> APRKARTAFSDHQLNQLERSFERQKYLSVQDRMDLAAALNLTDTQVKTWYQNRRTKWKRQTAVG;> KKPRKARTAFSDHQLNQLERSFERQKYLSVQDRMDLAAALNLTDTQVKTWYQNRRTKWKRQTA

However, analyses of the formation of TF complexes on DNA have revealed that many TFs also bind together across the family boundaries, in a DNA-dependent or DNA-facilitated manner. Because the DNA-bound TFs are fixed at particular positions relative to each other, the contact surfaces required for cooperative DNA-facilitated binding are very small, and can evolve rapidly. We also generated an unseen test set by solving six structures that represent several TF–TF–DNA complexes bound to optimal DNA sequences. The structures included two BARHL2 homodimers with two spacings, HOXB13 homodimer and TEAD4–HOXB13, MEIS1–HOXB13 and FOXK1–ELF1 heterodimers.

Recently released versions of RoseTTAFold (RoseTTAFold2NA v.0.2)39 and AlphaFold (AlphaFold v.3.0), which can predict the structures of protein–nucleic acid complexes, performed much better in predicting the overall geometry of TF–TF–DNA complexes. For example, both RoseTTAFold2NA and AlphaFold 3 correctly predicted the two homodimers of BARHL2. However, they still failed in most cases to correctly predict preferred spacings and orientations of TF–TF pairs bound to DNA, owing potentially to their inability to predict key TF–TF and TF–DNA contacts that depend on the orientation and spacing of the TF pairs.> EVRRILPADIKREVLIKDENAETNPDWGFPPEKRPIEMHIQFGVINLDKPPGPTSHEVVAWIKKILNLEKAGHGGTLAPKVSGVLPVALEKATRVVQALLPAGKEYVALMHLHGDVPEDKIIQVMKEFEGEIIQRPPLRSAVKRRLRTRKVYYIEVLEIEGRDVLFRVGVEAGTYIRSLIHHIGLALGVGAHMSELRRTRSGPFKEDETLITLHDLVDYYYFWKEDGIEEYFRKAIQPMEKAVEHLPKVWIKDSAVAAVTHGADLAVPGIAKLHAGIKRGDLVAIMTLKDEL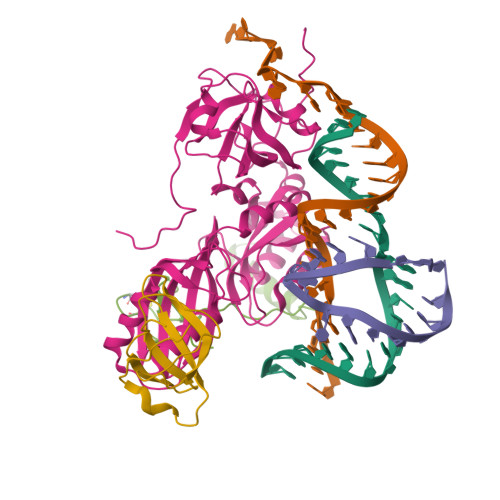VALGKAMMTSQEMLEKTKGIAVDVEKVFMPRDWYPKLWEKRD;> FRIRKCPKCGRYTLKEVCPVCGEKTKVAHPPRFSPEDPYGEYRRRWKREVLGI;> MKRLGKVLHYAKQGFLIVRTNWVPSLNDRVVDKRLQFVGIVKDVFGPVKMPYVAIKPKVSNPEIYVGEVLYVDE> AKCVSYGVSQIKAPALHSQGYTGSNVKVAVIDSGIDSSHPDLNVAGGASFVPSETNPFQDNNSHGTHVAGTVLAVAPSASLYAVKVLGADGSGQYSWII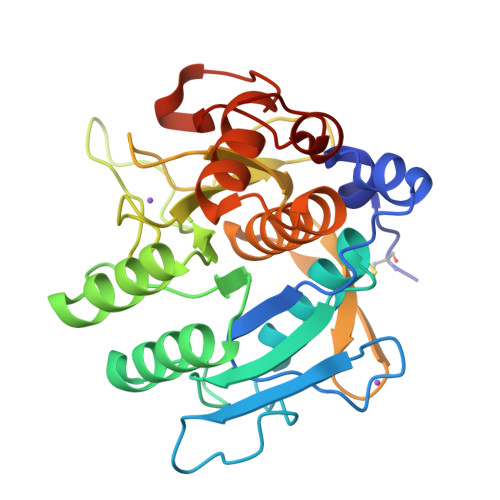NGIEWAIANNMDVINMSLGGPSGSAALKAAVDKAVASGVVVVAAAGNSGTSGSSSTVSYPAKYPSVIAVGAVDSSNQRAPFSSVGPELDVMAPGVSICSTLPGNKYGAHSGTCPASNHVAGAAALILSKHPNWTNTQVRSSLENTATKLGDSFYYGKGLINVEAAAQHHHHHH> MSEGFSSSSIQELYQSLKEITNNADVELFEDRITKLDFESTDEPKHANDIIKDRFLRPSNALPWSLLDMVQDVPHTSSPEDCSGKLDYKELLKVPDPINRTSYQFKRTGLEGKISGYKEEVDLKEVANANASNSLSITRSINHNQNSVRGSTAQLPFTPGGIPMKSVKTDSEQNGSSTMANATKLLHKDGQGLFDIPEGMNRGIKPMDSPAENEDQNGQFKELKQLNEIDNELDIRIEANEAKLKEEEKSAKSISEEIMEEATEETTADNADDAEIDELLPIGIDFGRTKPVSKSVPVKKEWAHVVDLNHKIENFDELIPNPARSWPFELDTFQKEAVYHLEQGDSVFVAAHTSAGKTVVAEYAIAMAHRNMTKTIYTSPIKALSNQKFRDFKETFDDVNIGLITGDVQINPDANCLIMTTEILRSMLYRGADLIRDVEFVIFDEVHYVNDQDRGVVWEEVIIMLPQHVKFILLSATVPNTYEFANWIGRTKQKNIYVISTPKRPVPLEINIWAKKE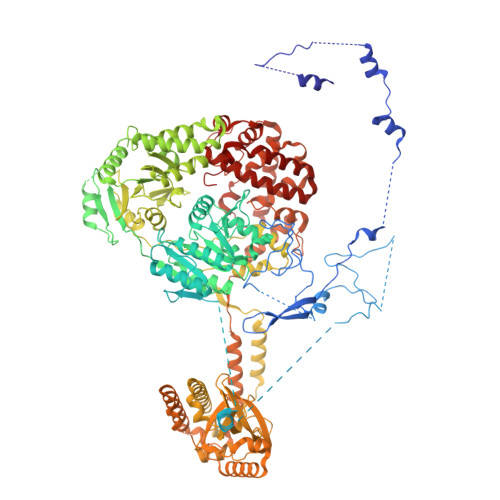LIPVINQNSEFLEANFRKHKEILNGESAKGAPSKTDNGRGGSTARGGRGGSNTRDGRGGRGNSTRGGANRGGSRGAGAIGSNKRKFFTQDGPSKKTWPEIVNYLRKRELLPMVVFVFSKKRCEEYADWLEGINFCNNKEKSQIHMFIEKSITRLKKEDRDLPQILKTRSLLERGIAVHHGGLLPIVKELIEILFSKGFIKVLFATETFAMGLNLPTRTVIFSSIRKHDGNGLRELTPGEFTQMAGRAGRRGLDSTGTVIVMAYNSPLSIATFKEVTMGVPTRLQSQFRLTYNMILNLLRIEALRVEEMIKYSFSENAKETLQPEHEKQIKVLQEELQTIEYKSCEICDNDIEKFLELMLAYKEATVNLMQEMVKSPSILHILKEGRLVAFRDPNDCLKLGFVFKVSLKDAVCVIMTFTKPYKLPNGEPNHLIYFPKADGYRRRNFPKFQKTDFYMEEVPVTAIEVITKRKFAAPLGKVIKKDVAALNEFNAETNNILDGKTLKEAINIEKQGLKIHQILLDRTNIRDEIFKLKSIKCPNLSQHIVPKFKAHVIKKKIEELYHLMSDQNLSLLPDYEKRLAVLKDTEFIDQNHNVLLKGRVACEINSGYELVLTELILDNFLGSFEPEEIVALLSVFVYEGKTREEEPPIVTPRLAKGKQRIEEIYKKMLCVFNTHQIPLTQDEAEFLDRKRFAMMNVVYEWARGLSFKEIMEMSPEAEGTVVRVITWLDEICREVKTASIIIGNSTLHMKMSRAQELIKRDIVFAASLYL> MNFGVEDMIEHVPMEDK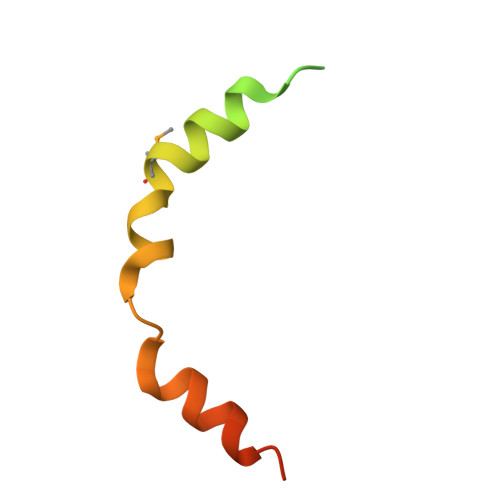RKGAAALDEARLRQQAIGVKLRQMFDEVVNEPVPDEFLAILRKAERPAGGE dihydroxyacetic acid | C2 H4 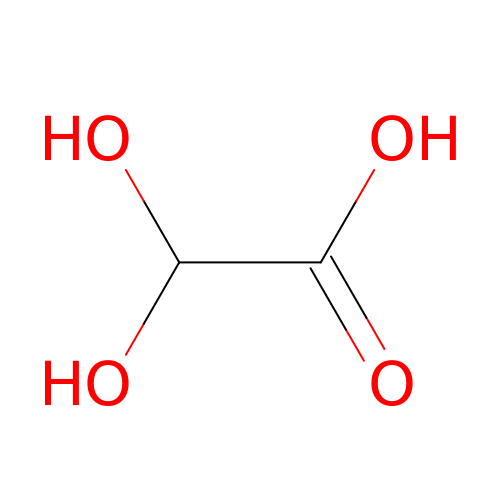O4 | GOCCREQJUBABAL-UHFFFAOYSA-N> SASPAVAELCQNTPETFLEASKLLLTYADNILRNPSDEKYRSIRIGNTAFSTRLLPVRGAVECLFEMG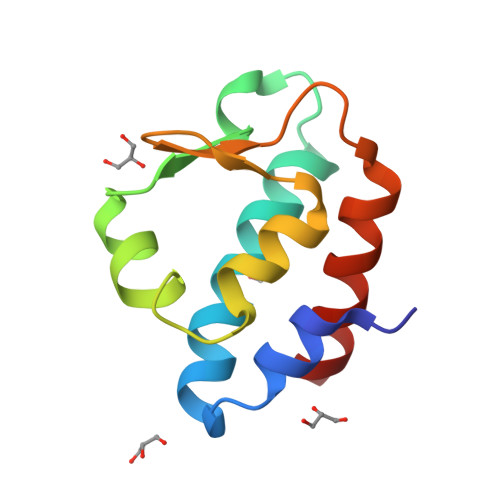FEEGETHLIFPKKASVEQLQKIRDLIAIERS> MWENLWYLDILINVLIITI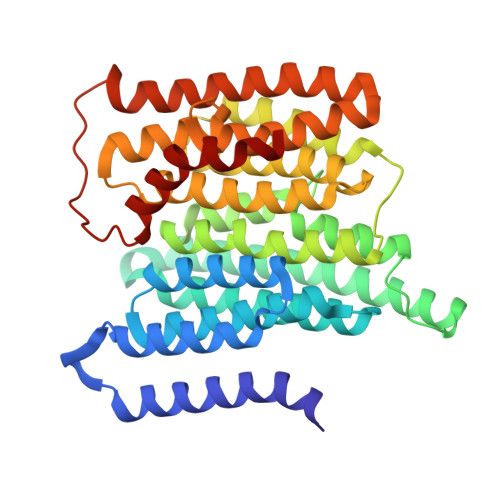FGLISCSSSATKSYDLKGCFIISMVGGVYDIPSAILWCLASLSILNFNGFFASLFLVFTWISNLFAMQSLNFLGIYLAFEMQSLCLLVLGKITANENQRWFAYRGLLKYLVLSLIAGSIFIFHASSSYLQSGVMISDSLVTYVFLLFKLGVAPFHMYTLELFSVVSRHVAFVFSTLPKLSVLYLISNSNIGSECVWWGLISLWLGSISQYQSVFVRSILLYSSVAEIGLVLLVLQEGFSWEAFSWVSIYFLSLSGVWHANSKFVSAISVASIAGLPPFLGFIGKAQILKSLVSINLGILIFSSILAATISFIGYLRLIRLMYLVSPVKWKNNKDSSFINWSTWMLTVGTLPMVYSV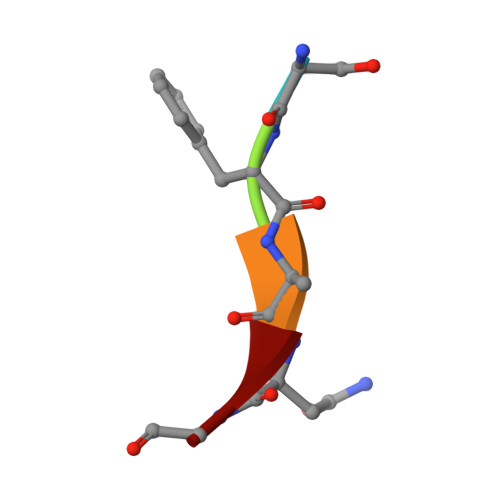> SFANG(S)-10-((2S,3S,4R)-5-((S)-((S)-(((2R,3S,4R,5R)-5-(6-AMINO-9H-PURIN-9-YL)-3,4-DIHYDROXY-TETRAHYDROFURAN-2-YL)METHOXY)(HYDROXY)PHOSPHORYLOXY)(HYDROXY)PHOSPHORYLOXY)-2,3,4-TRIHYDROXYPENTYL)-7,8-DIMETHYL-2,4-DIOXO-2,3,4,4A-TETRAHYDROBENZO[G]PTERIDINE-5(10H)-SULFONIC 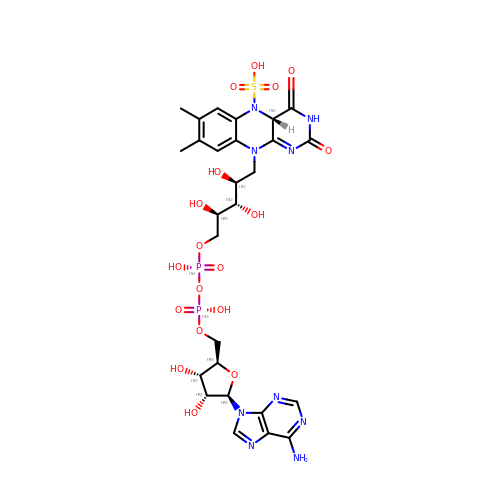ACID | C27 H35 N9 O18 P2 S | WCBOBURWKHIISA-LDVRFEIFSA-N> MTEHETKDKAKKIREIYRYDEMSNKVLKVDKRFMNTSQNPQRDAEISQPKSMSGRISAKDMGQGLCNNINKGLKENDVAVEKTGKSASLKKIQQHNTILNSSSDFRLHYYPKDPSNVETYEQILQWVTEVLGNDIPHDLIIGTADIFIRQLKENEENEDGNIEERKEKIQHELGINIDSLKFNELVKLMKNITDYETHPDNSNKQAVAILADDEKSDEEEVTEMSNNANVLGGEINDNEDDDEEYDYNDVEVNSKKKNKRALPNIENDIIKLSDSKTSNIESVPIYSIDEFFLQRKLRSELGYKDTSVIQDLSEKILNDIETLEHNPVALEQKLVDLLKFENI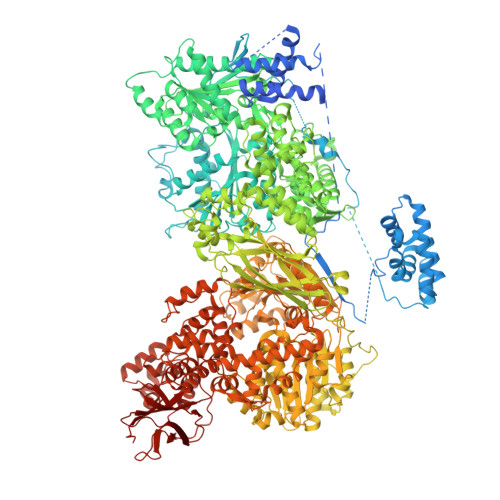SLAEFILKNRSTIFWGIRLAKSTENEIPNLIEKMVAKGLNDLVEQYKFRETTHSKRELDSGDDQPQSSEAKRTKFSNPAIPPVIDLEKIKFDESSKLMTVTKVSLPEGSFKRVKPQYDEIHIPAPSKPVIDYELKEITSLPDWCQEAFPSSETTSLNPIQSKVFHAAFEGDSNMLICAPTGSGKTNIALLTVLKALSHHYNPKTKKLNLSAFKIVYIAPLKALVQEQVREFQRRLAFLGIKVAELTGDSRLSRKQIDETQVLVSTPEKWDITTRNSNNLAIVELVRLLIIDEIHLLHDDRGPVLESIVARTFWASKYGQEYPRIIGLSATLPNYEDVGRFLRVPKEGLFYFDSSFRPCPLSQQFCGIKERNSLKKLKAMNDACYEKVLESINEGNQIIVFVHSRKETSRTATWLKNKFAEENITHKLTKNDAGSKQILKTEAANVLDPSLRKLIESGIGTHHAGLTRSDRSLSEDLFADGLLQVLVCTATLAWGVNLPAHTVIIKGTDVYSPEKGSWEQLSPQDVLQMLGRAGRPRYDTFGEGIIITDQSNVQYYLSVLNQQLPIESQFVSKLVDNLNAEVVAGNIKCRNDAVNWLAYTYLYVRMLASPMLYKVPDISSDGQLKKFRESLVHSALCILKEQELVLYDAENDVIEATDLGNIASSFYINHASMDVYNRELDEHTTQIDLFRIFSMSEEFKYVSVRYEEKRELKQLLEKAPIPIREDIDDPLAKVNVLLQSYFSQLKFEGFALNSDIVFIHQNAGRLLRAMFEICLKRGWGHPTRMLLNLCKSATTKMWPTNCPLRQFKTCPVEVIKRLEASTVPWGDYLQLETPAEVGRAIRSEKYGKQVYDLLKRFPKMSVTCNAQPITRSVMRFNIEIIADWIWDMNVHGSLEPFLLMLEDTDGDSILYYDVLFITPDIVGHEFTLSFTYELKQHNQNNLPPNFFLTLISENWWHSEFEIPVSFNGFKLPKKFPPPTPLLENISISTSELGNDDFSEVFEFKTFNKIQSQVFESLYNSNDSVFVGSGKGTGKTAMAELALLNHWRQNKGRAVYINPSGEKIDFLLSDWNKRFSHLAGGKIINKLGNDPSLNLKLLAKSHVLLATPVQFELLSRRWRQRKNIQSLELMIYDDAHEISQGVYGAVYETLISRMIFIATQLEKKIRFVCLSNCLANARDFGEWAGMTKSNIYNFSPSERIEPLEINIQSFKDVEHISFNFSMLQMAFEASAAAAGNRNSSSVFLPSRKDCMEVASAFMKFSKAIEWDMLNVEEEQIVPYIEKLTDGHLRAPLKHGVGILYKGMASNDERIVKRLYEYGAVSVLLISKDCSAFACKTDEVIILGTNLYDGAEHKYMPYTINELLEMVGLASGNDSMAGKVLILTSHNMKAYYKKFLIEPLPTESYLQYIIHDTLNNEIANSIIQSKQDCVDWFTYSYFYRRIHVNPSYYGVRDTSPHGISVFLSNLVETCLNDLVESSFIEIDDTEAEVTAEVNGGDDEATEIISTLSNGLIASHYGVSFFTIQSFVSSLSNTSTLKNMLYVLSTAVEFESVPLRKGDRALLVKLSKRLPLRFPEHTSSGSVSFKVFLLLQAYFSRLELPVDFQNDLKDILEKVVPLINVVVDILSANGYLNATTAMDLAQMLIQGVWDVDNPLRQIPHFNNKILEKCKEINVETVYDIMALEDEERDEILTLTDSQLAQVAAFVNNYPNVELTYSLNNSDSLISGVKQKITIQLTRDVEPENLQVTSEKYPFDKLESWWLVLGEVSKKELYAIKKVTLNKETQQYELEFDTPTSGKHNLTIWCVCDSYLDADKELSFEINVK> MTRRYLKYYIFVTLLFFVQVINNVLCAPDNKQEQGKYLNRTINILNAGKNIAKSYGHNKLKPIHILSALAKSDYGSTLFKENNVNAANLKEYIDIALEQTRAGAPLDNKSKIVNSAEVKETLALAEAAANKY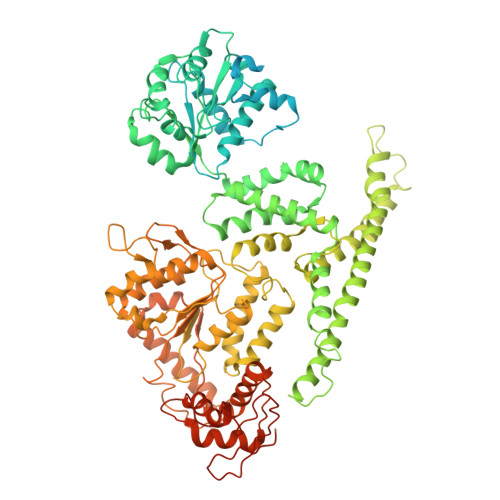KSPKVDVEHLLSGLSNDELVNEIFNEVYLTDEAIKAILKRKFEKTKKDKDGKTGTLYIEQFGSNMNEKVRNGKLQGIYGRDEEIRAIIESLLRYNKNSPVLVGNPGTGKTTIVEGLVYRIEKGDVPKELQGYTVISLNFRKFTSGTSYRGEFETRMKNIIKELKNKKNKIILFVDEIHLLLGAGKAEGGTDAANLLKPVLSKGEIKLIGATTIAEYRKFIESCSAFERRFEKILVEPPSVDMTVKILRSLKSKYENFYGINITDKALVAAAKISDRFIKDRYLPDKAIDLLNKACSFLQVQLSGKPRIIDVTERDIERLSYEISTLEKDVDKVSKKKYNKLIKEFEEKKEQLKKYYEEYVITGERLKRKKEIEKKLNDLKELTQNYVYSNKEPPIELQNSLKEAQQKYLELYKETVAYVEAKTHNAMNVDAVYQEHVSYIYLRDSGMPLGSLSFESSKGALKLYNSLSKSIIGNEDIIKSLSDAVVKAATGMKDPEKPIGTFLFLGPTGVGKTELAKTLAIELFNSKDNLIRVNMSEFTEAHSVSKITGSPPGYVGFSDSGQLTEAVREKPHSVVLFDELEKAHADVFKVLLQILGDGYINDNHRRNIDFSNTIIIMTSNLGAELFKKKLFFDADNSGTPEYKRVMEDVRLSLIKKCKKVFKPEFVNRIDKIGVFEPLNKKNLHKIVALRFKKLEKRLEEKNIQVSVSEKAIDYIIDQSYDPELGARPTLIFIESVIMTKFAIMYLKKELVDDMDVFVDYNSKAKNLVINLSKTPRDYKDDDDKDYKDDDDKDYKDDDDK The OBV M segment encodes two glycoproteins, Gn and Gc, derived from a single polyprotein precursor, with Gn encoded upstream of Gc. Compared with other bunyaviruses, OBV Gn is relatively small, with an ectodomain of about 200 amino acids (aa), whereas Gc, with an ectodomain of ca. 900 aa long, is about twice the size of its Gc counterparts from other bunyaviruses. Our structural analysis has revealed that this region is composed of two domains: a 27 -kDa α-helical head domain and a stalk that is divided into two identically folded 19 -kDa tandem β-sandwiches. Furthermore, the head domain is well exposed to the environment and is a major target of the humoral adaptive immune system of the OBV mammalian hosts, indicating that the trigonal pyramid of the spike shields the functionally more critical membrane fusion core machinery from the host’s antibody response.

We crystallized the N-terminal half of SBV Gc (aa 465–874 in the glycoprotein precursor) produced in recombinant Drosophila S2 cells. The best crystals diffracted anisotropically to 2.5–2.0 Å resolution, which allowed the X-ray structure determination and refinement to a final Rfree value of 0.24. The structure showed two rigid domains separated by a hinge, adopting a V-shaped conformation in the crystal. The N-terminal head domain (aa 465–702) constitutes the first arm of the V. It is an α-helical bundle with approximate dimensions of 6.5 × 4.0 × 3.5 nm in size with a molecular mass of 27 kDa. It is internally stabilized by four disulfide bonds and carries two N-linked carbohydrate chains at positions N493 and N686, protruding from the same face of the ellipsoidal head domain. Of note, the glycan chain attached to N493, which was earlier shown to be essential for protein folding and secretion, is well ordered through stabilization by the local protein environment and not by crystal packing. The rod-shaped second domain, which we term stalk (see below), has dimensions of 7.0 × 3.0 × 2.5 nm and extends from the vertex of the V-shaped molecule. The stalk can be further divided into two subdomains (aa 703–798/ 799–874). Despite having low aa sequence identity (18%) with each other, the two stalk subdomains share a common fold with a root-mean-square deviation (RMSD) of 3.2 Å over 64 Cα atoms, indicating that they derive from gene duplication. Each stalk subdomain has a molecular mass of ~19 kDa and comprises two antiparallel β sheets packing against each other. Moreover, each stalk subdomain is internally stabilized by three conserved disulfide bonds, with the corresponding cysteine residues conserved between them and across OBVs.

>[2x]EWSHPQFEKGGQETSINCKNIQSTQLTIEHLSKCMAFYQNKTSSPVVINEIISDASVDEQELIKSLNLNCNVIDRFISESSVIETQVYYEYIKSQLCPLQVHDIFTINSASNIQWKALARSFTLGVCNTNPHKHICRCLESMQMCTSTKTDHAREMSIYYDGHPDRFEHDMKIILNIMRYIVPGLGRVLLDQIKQTKDYQALRHIQGKLSPKSQSNLQLKGFLEFVDFILGANVTIEKTPQTLTTLSLIKGAHRNLDQKDPGPTPILVCKSPQKVVCYSPRGVTHPGDYISCKSKMYKWPSLGVYKHNRDQQQACSSDTHCLEMFEPAERTITTKICKVSDMTYSESPYSTGIPSCNVKRFGSCNVRGHQWQIAECSNGLFYYVSAKAHSKTNDITLYCLSANCLDLRYAFRSSSCSDIVW> MPEITRRRALTAAAAVAATASAAVTLAAPAASAAGHHEPAAPESFDEVYKGRRIQGRPARGAAHHHEHGGGYEVFVDGVQL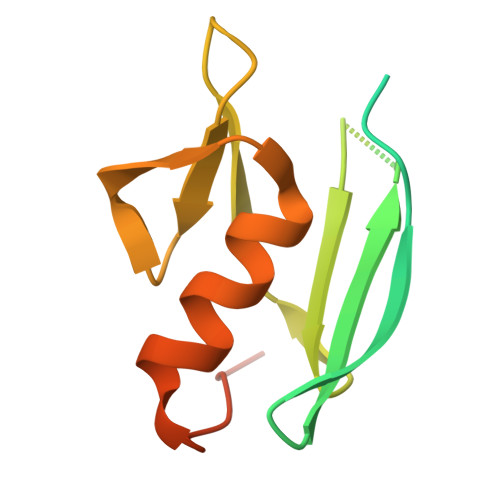HVMRNADGSWISVVSHYDPVPTPRAAARAAVDELQGAPLLPFPANLEHHHHHH>MNHKVHMMSQPKPILYYDERSPPVRSCLMLIKLLDIDVELRFVNLFKGEQFQKDFLALNPQHSVPTLVHGDLVLTDSHAILIHLAEKFDEGGSLWPQEHAERMKVLNLLLFECSFLFRRDSDFMSAIVRQGFANVDVAHHERKLTEAYIIMERYLENSDFMAGPQLTLADLSIVTTLSTVNLMFPLSQFPRLRRWFTAMQQLDAYEANCSGLEKLRQTMESVGSFQFPSSSAVVTEKVE[2x]

Here, we report the first crystal structure of an ecdysteroidogenic regulator encoded by the Halloween gene, noppera-bo (nobo). nobo encodes a member of the epsilon class of cytosolic GSH S-transferases (GST, EC 2.5.1.18; hereafter GSTEs). DmNobo forms a polypeptide homodimer with a canonical GST fold, which has a well-conserved GSH-binding site (G-site) and a hydrophobic substrate-binding pocket (H-site) adjacent to the G-site. Consistent with the requirement of GSH for GST function, a defect in GSH biosynthesis in D. melanogaster also leads to larval lethality, which is partly rescued by the administration of 20E or cholesterol. These data indicate that the nobo family of GSTs is essential for ecdysteroid biosynthesis by regulating cholesterol trafficking and/or metabolism. In general, GSTs catalyze various reactions with an activated glutathione (GSH) molecule in the following three ways: GSH conjugation to a substrate, reduction of a substrate using GSH, and isomerization.

GSH and EST binding did not affect the overall structure of DmNobo; the root mean square deviation (RMSD) values for each pair among the four crystal structures were comparable with respect to the estimated coordinate errors.> MAAAGSLYWRTSRELWTILLGRSSMKDGYQIKAELDRYGDRLLQGLAYYKPPSTRSADKVKANKNLSPALQELGLRLSKFLALDEEQSVELLQTYLQYDYRGTQESVKVLPQDERQSQALMLKMADYYYEERISLLRCVLYILNYFQDDKHPYSAEFSKCVELMEQKELFGKYLKQFESLCREEAPTWETHGNFMTERQVSRWFVQRLREQAMLLEIIFLYFACFAASPSDLLALTKLFKEQGFGCRLQNHHLVEPSMDPLVERIGYFSILIFLEALDMDTLMTCSLSDKIEQHPFSSEEQVCKEMDSILVTLGDVPHHGPVLLAWALLRFTLNPDKVTSAVRKMGSTAIQLHLFQYLTRMLQSLRSGENNCTTSTACLCVYTFLAYVLSTLEEQVSQSQQDLVETACQVFAAPNLPDLFWNMEPTAGLGILLDSVVGMFPFRISPLLKLFTALVSKSSAKKVYSFLDRMSSYTEHYRHKPHDILSHDDETLWKRQTPKLLYALGLGQTNLRIPQGALGQVMADENGFLVRWEYSYSCWTLFTCEIEMLLHVVSTADVIHQCQRVKPIIDLVHKVISTDLSIADCLLPITSRIYMLLQRLTTVMNPPMDFLSSCVDCLTALATRLPAKVWTDLRHTGFLPFAANPVSGHLISTEGMNAGGYGSLFGIEQSQGEYSVTLSFLRLITTLVKGQLGSTQSQGLVPCILFVLREMLPNYHRWRYNSHGVREQLGFQILSLIHAILNLCPEEEEGSSAPNLRSLCIFSLTNTEAGQAVINIMGIGVDTLNTVML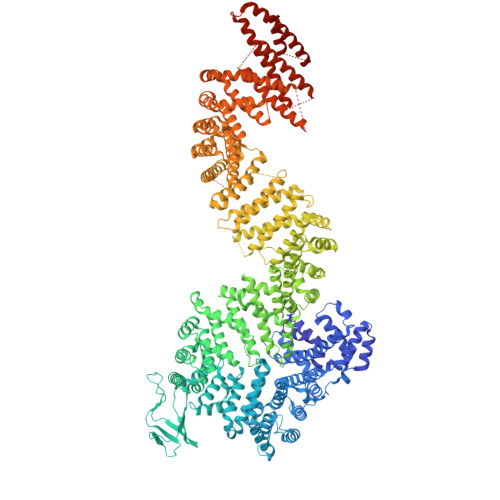TQAGSSGTEGQGQMLMQTIKLAFSITNNVIRLKPPSSGVSPLEHALTQHGAHGNNLIAVLAKYIYHRYDPSLPRLAIQLLKRLAMVAPMSVYACLGSDAAAIRDAFLSRLRDNIEDMQIKIMILEFLTVAVETQPGLIELFLNLEAKDTNEGSKEYSLGEWSCLQVVLKLIDSQDPESSWGAPLLHRSAIAFLHALWQDRRDSAMTVLRTKPNFWENLTSPLFGTLACPSESSELSILETCAFIMKIICLEIYYAVRGSLGDSLKKILKKFSEEERFTYWSNYVHSLVCQVAETEGTCNSLTEYQQLLSAWRMFLIVATHNADVMHLTNPEVRQKLFKDILGGTQALLVVPRSVACMHLSSMLCTVMIILLRRWKNDLAAPEDILNSLTQILEGVLQRDQQLVEKTKAQIFSALISVLEMKPMKASEIPQYSQLLLNVCETLQEEVVSLVDHTRHEVPASDTSEDKDSMETEDTGRIRQKDQRDGVCVLGLHLAKELCEADEEGDQWQQVLRKLPVLPILFSALEVSLRIKQNLHFCEAILHFLFTLAKTHQGAAAMAGAGITQTVCLPLLSVYQLSSNGAGSVQPAVSLRKSLDAPSWPGVYRLTVSLMERLLKTLRYNFLSEALDFVGVHQERILQCLSAVRTVQSLSCLEEADHTVGFLLQLSNFTKEWHFHLPQLIKDVQVNLCYLCQACTSLLHSRKMLQHYLQIKNGESMSSTATPRGQRTPQTPSKQPTAESEALELRQLRTVQHSLLKILGKTLATLRAFTPDLCQILQVQPLDLAQYNLLFALSFTTPAFDADVTPSFGTLLATVNVTLSMLGEMDKKKDHPLSRALVESNNTGESKNNKSLLLFIMENCFYLLISQAVRYLRDPSVHPRDKQRMKQELSSELSTLLSSLSRYFRRGGPSSPAGGLMPSPQPKGASAAKVVPEAQEPLIQLVQAFVRHVQR> MAKKHKCPECPAGEKWAVPYADFLSLLLALFIALWAISKTNPAKVEALKTEFVKIFDYTSTQTVKEESKTQEKYKGA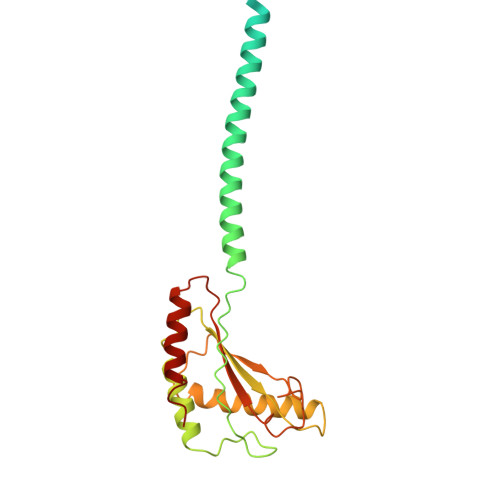AKEESDELKSLKQMTMTQQETIKRLQAALDQSDNQVALNLPSKVEFERGSAQIVSADIQDYLKRMAELTTYLPPQAKIEIRGYTDNSDSIIRSYELAYQRAENVLKYFIEGGANLKNISIKSYGLNNPINGNPQALENNRVEIYFKVDTADTSTQKSVLELINKIGTKAP Cystargolide A (bound) | 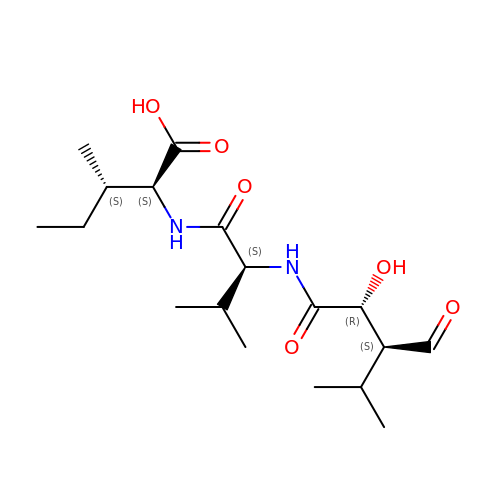C18 H32 N2 O6 | NPCIMWWVLQVJPA-YYFQZIEXSA-N The fold of CrataBL consists of a β-trefoil, typical for this protein family. To conclude, the sequence and three-dimensional structure of CrataBL show extensive similarity to protease inhibitors of the Kunitz-type, although the inhibitory activity is weak (in the micromolar range). A number of its biological properties have been characterized, including delay in clot formation by impairing the intrinsic pathway of coagulation cascade. In addition, CrataBL was shown to exhibit anti-inflammatory, analgesic, insecticidal, and anti-tumor activities.

The three-dimensional structure of CrataBL was determined in two crystal forms. Both of them were in space group C2 and contained two molecules in the asymmetric unit, but the unit cell parameters and crystal packing were different. Further analysis of glycosylation by mass spectrometry and protein sequence determination has shown the presence of N-linked oligosaccharides at Asn27 and Asn57. However, it is not clear whether the dimer observed in both crystal forms of CrataBL is biologically significant. There is no particular need for dimerization of a protease inhibitor, since Kunitz-P type inhibitors form 1∶1 complexes with their target enzymes. Since we were not able to obtain crystals of CrataBL with a target protease such as trypsin, the location of the reactive loop may only be predicted. However, the observation that CrataBL is slowly cleaved by trypsin between serines 58 and 59, located on a loop that is involved in direct interaction with the active site residues in trypsin and other serine proteases, lends credence to this assumption. Thus the detailed structural basis of the inhibition mode by CrataBL still needs to be verified.

>AILTGVPYYILPSTSRAGFSPDNLRKNTSQPSCPLDLITQLRFPPRIGVPVIFTPQNSSLKVVPLSHNLNIHTCSDLWFCPESKIWTVKSSSIHRGLVVTTGGTFRSLGSWFRIERHGDSYKLVHCPRGSTPCRDVGIETVGGGGRRYLAPRDRPLAVRFTRASG[2x]>[2x]GSMGKDEALEKDL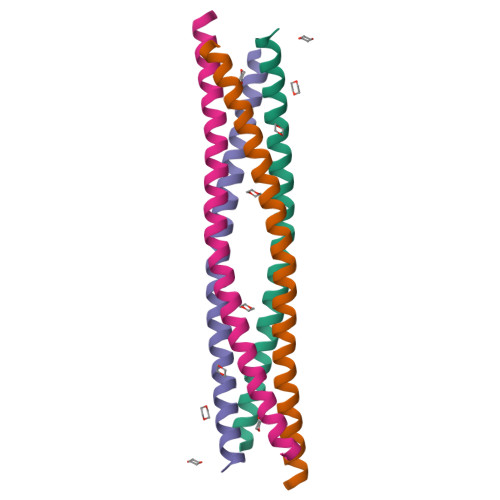NDVSKEINLMLSTYAKLLSERAAVDASYIDEIDELFKEANAIENFLIQKREFLRQR> Y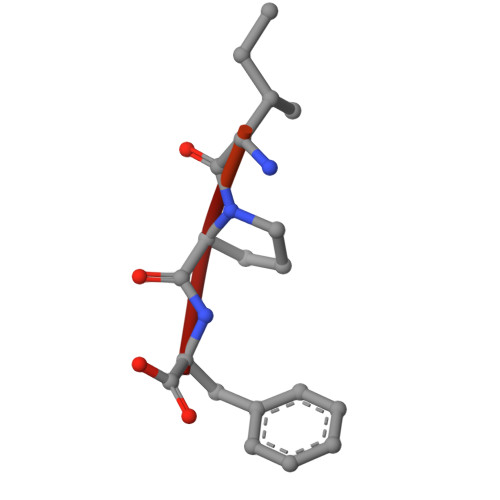MDFDDDIPF>[4x]MNLQRFPRYPLTFGPTPIQPLARLSKHLGGKVHLYAKREDCNSGLAFGGNKTRKLEYLIPEALAQGCDTLVSIGGIQSNQTRQVAAVAAHLGMKCVLVQENWVNYSDAVYDR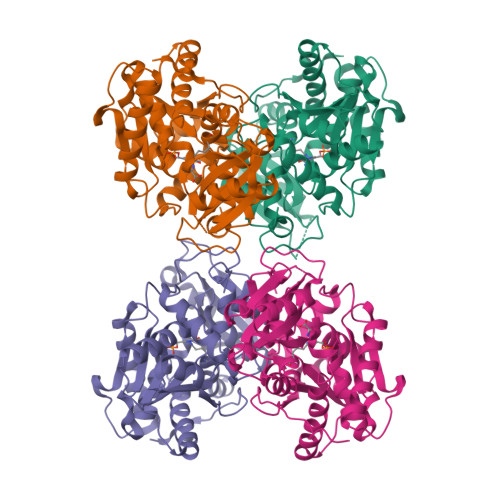VGNIQMSRILGADVRLVPDGFDIGFRRSWEDALESVRAAGGKPYAIPAGCSDHPLGGLGFVGFAEEVRAQEAELGFKFDYVVVCSVTGSTQAGMVVGFAADGRADRVIGVDASAKPAQTREQITRIARQTAEKVGLERDIMRADVVLDERFAGPEYGLPNEGTLEAIRLCARTEGMLTDPVYEGKSMHGMIEMVRNGEFPEGSRVLYAHLGGVPALNGYSFIFRDG> MSMAEMLRRDEGLRLKVYWDTEGYPTIGIGHLIMKQPVRDMAQINKVLSKQVGREITGNPGSITMEEATTLFERDLADMQRDIKSHSKVGPVWQAVNRSRQMALENMAFQMGVGGVAKFNTMLTAMLAGDWEKAYKAGRDSLWYQQTKGRASRVTMIILTGNLESYGVELEHHHHHH;> MKKFIFATIFALASCAAQPAMAGYDKDLCEWSMTADQTEVETQIEADIMNIVKRDRPEMKAEVQKQL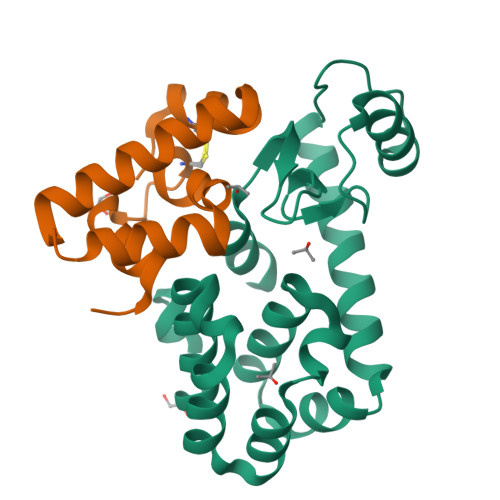KSGGVMQYNYVLYCDKNFNNKNIIAEVVGELEHHHHHH> GPHMREYKLVVLGSGGVGKSALTVQFVQGIFVEKYDPTIEDSYRKQVEVDAQQCMLEILDTAGTEQFTAMR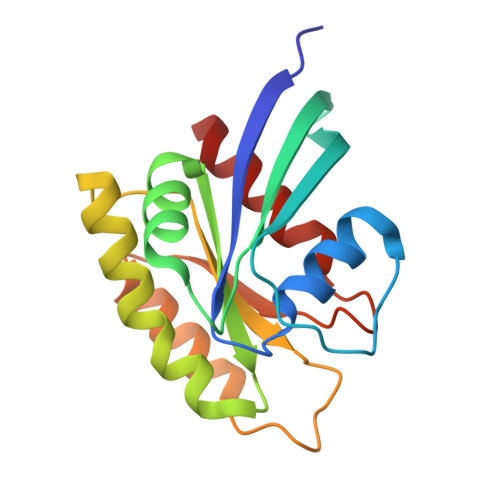DLYMKNGQGFALVYSITAQSTFNDLQDLREQILRVKDTDDVPMILVGNKCDLEDERVVGKEQGQNLARQWNNCAFLESSAKSKINVNEIFYDLVRQINR>MKVLSYLKNFYLFLAIGAIMQASENMGSQHQKTDERVIYLAGGSFWGLEAYMERIYGVIDASSGYANGKTSSTNYEKLHESDHAESVKVIYDPKKISLDKLLRYYFKVVDPVSVNKQGNDVGRQYRTGIYYVNSADKEVIDHALKALQKEVKGKIAIEVEPLKNYVRAEEYHQDYLKKHPSGYCHIDLKKADEVIVDDDKYTKPSDEVLKKKLTKLQYEVTQNKHTEKPFENEYYNKEEEGIYVDITTGEPLFSSADKYDSGCGWPSFSKPINKDVVKYEDDESLNRKRIEVLSRIGKAHLGHVFNDGPKELGGLRYSINSAALRFIPLKDMEKEGYGEFIPYIKKGELKKYINDKKSH[2x]

Methionine sulfoxide reductase (Msr) is a family of enzymes that reduces oxidized methionine and plays an important role in the survival of bacteria under oxidative stress conditions. MsrA is stereospecific for reducing L-methionine S-sulfoxide, whereas MsrB is stereospecific for the reduction of the R diastereomer. MsrA and MsrB exist in a fusion protein form (MsrAB) in some pathogenic bacteria, such as Helicobacter pylori (Hp), Streptococcus pneumoniae, and Treponema denticola. The catalytic activities of the MsrAB fusion protein are higher than those of the individual enzymes, MsrA and MsrB.

The crystal structure of HpMsrABC44S/C318S was solved at 2.2 Å and belonged to the P1 space group. There were two protomers (MolA and MolB) in the asymmetric unit. Each monomer of HpMsrABC44S/C318S had two catalytic domains, HpMsrA (34–192, residue number) and HpMsrB (206–357), which were linked by the linker region, iloop (193–205). To understand the fused form instead of the separated enzyme at the molecular level, we determined the crystal structure of HpMsrABC44S/C318S at 2.2 Å, which showed that a linker region (Hpiloop, 193–205) between two domains interacted with each HpMsrA or HpMsrB domain via three salt bridges (E193-K107, D197-R103, and K200-D339). Even though we co-crystallized an HpMsrAB mutant (C44S/C318S) protein with the substrate analog compound, dabsyl-Met-(R,S)-O, no analog compounds were found in the active sites of HpMsrA or HpMsrB. We found two acetate molecules in the active site pocket, which was used as the crystallization buffer (0.1 M sodium acetate). In the active site of the HpMsrA domain, the carboxyl group of the acetate ion interacted with Oδ1 of E85 (2.50 Å), OH of Y75 (2.60 Å), OH of Y125 (2.79 Å), and Oδ of S44 (2.93 Å). The interaction residues were as follows: the carboxyl group of the acetate ion interacted with Nε of H303 (2.69 Å), one water molecule (W4, 2.70 Å), and Oδ of C318S (2.67 Å). Therefore, both the active sites of HpMsrAB were reduced. In addition, we found that the linker region (Hpiloop) connecting HpMsrA and HpMsrB was mandatory for the higher catalytic efficiency of HpMsrAB based on biochemical and kinetic analyses.> NPVERYVDEVLNEVLVVPNINQSHPTTSNAAPVLDAAETGHTNKIQPEDTIETRYVQSSQTLDEMSVESFLGRSGCIHESVLDIVDNYNDQSFTKWNINLQEMAQIRRKFEMFTYARFDSEITMVPSVAAKDGHIGHIVMQYMYVPPGAPIPTTRDDYAWQSGTNASVFWQHGQPFPRFSLPFLSIASAYYMFYDGYDGDTYKSRYGTVVTNDMGTLCSRIVTSEQLHKVKVVTRIYHKAKHTKAWCPRPPRAVQYSHTHTTNYKLSSEVHNDVAIRPRTNLTTV;> SDRIIQITRGDSTITSQDVANAVVGYGVWPHYLTPQDATAIDKPTQPDTSSNRFYTLDSKMWNSTSKGWWWKLPDALKDMGIFGENMFYHFLGRSGYTVHVQCNASKFHQGTLLVVMIPEHQLATVNKGNVNAGYKYTHPGEAGREVGTQVENEKQPSDDNWLNFDGTLLGNLLIFPHQFINLRSNNSATLIVPYVNAVPMDSMVRHNNWSLVIIPVCQLQSNNISNIVPITVSISPMCAEFSGARAKTVVQ;> GLPVYVTPGSGQFMTTDDMQSPCALPWYHPTKEIFIPGEVKNLIEMCQVDTLIPINSTQSNIGNVSMYTVTLSPQTKLAEEIFAIKVDIASHPLATTLIGEIASYFTHWTGSLRFSFMFCGTANTTLKVLLAYTPPGIGKPRSRKEAMLGTHVVWDVGLQSTVSLVVPWISASQYRFTTPD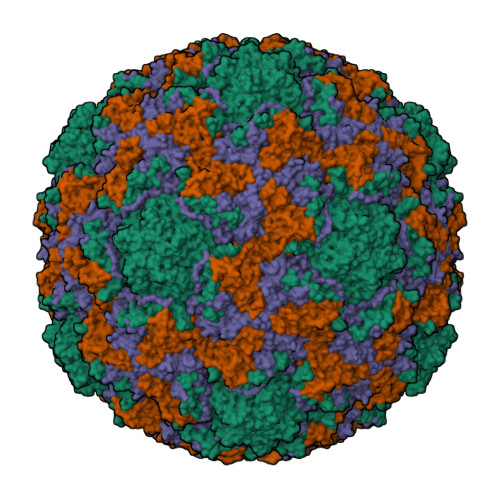TYSSAGYITCWYQTNFVVPPNTPNTAEMLCFVSGCKDFCLRMARDTDLHKQTGPITQ;> GAQVSRQNVGTHSTQNMVSNGSSINYFNINYFKDAASSGASRLDFSQDPSKFTDPVKDVLEKGIPTLQSPSVEACGY>[2x]SNAQTDPTGPEGPHLGQSRLFLLCHKEALMKRNFCVPPGASPEVPKPALSFYVLGSWLGGTQRKEGT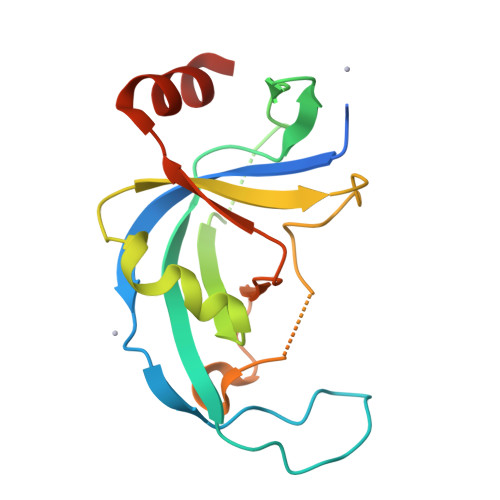GWGLPEPQGNDDNDQKVHLIFFGSSVRWFEFLHPGQVYRLIAPGPATPMLFEKDGSSCISRRPLELAGCASCLTVQDNWTLELESSQDIQDVLDANKSLPE>HHHHHHHHHHAQVNIAPGSLDKALNQYAAHSGFTLSVDASLTRGKQSNGLHGDYDVESGLQQLLDGSGLQVKPLGNNSWTLEPAPAPKEDALTVVGDWLGDARENDVFEHAGARDVIRREDFAKTGATTMREVLNRIPGVSAPENNGTGSHDLAMNFGIRGLNPRLASRSTVLMDGIPVPFAPYGQPQLSLAPVSLGNMDAIDVVRGGGAVRYGPQSVGGVVNFVTRAIPQDFGIEAGVEGQLSPTSSQNNPKETHNLMVGGTADNGFGTALLYSGTRGSDWREHSATRIDDLMLKSKYAPDEVHTFNSLLQYYDGEADMPGGLSRADYDADRWQSTRPYDRFWGRRKLASLGYQFQPDSQHKFNIQGFYTQTLRSGYLEQGKRITLSPRNYWVRGIEPRYSQIFMIGPSAHEVGVGYRYLNESTHEMRYYTATSSGQLPSGSSPYDRDTRSGTEAHAWYLDDKIDIGNWTITPGMRFEHIESYQNNAITGTHEEVSYNAPLPALNVLYHLTDSWNLYANTEGSFGTVQYSQIGKAVQSGNVEPEKARTWELGTRYDDGALTAEMGLFLINFNNQYDS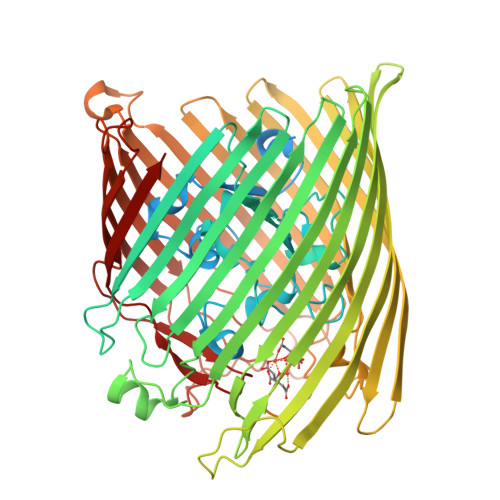NQTNDTVTARGKTRHTGLETQARYDLGTLTPTLDNVSIYASYAYVNAEIREKGDTYGNLVPFSPKHKGTLGVDYKPGNWTFNLNSDFQSSQFADNANTVKESADGSTGRIPGFMLWGARVAYDFGPQMADLNLAFGVKNIFDQDYFIRSYDDNNKGIYAGQPRTLYMQGSLKF[2x]>[2x]GPGGSPYLITGIPKDPKHPLPIRKDIDDWYLEQTSAGSNRIQLTLFVEALTVIQNRPLNDQLSYFRLAGIHGAPWTEWDGVPGGQKDSKGNPTGFAVHNNYTFPTWHRVYVTLYEQVIYEAMLDFIKQNVPQNGKADWENEAKQWRLPYWDFARFARHGHDNTQGDELRLPILVTMPMVKVLVPGQPGKQLSKPNPLYRFQMQTLMGTLERPYAITSQKTEEHGWSFDLPFDKCQSTTKYGLLENYNADVWADGGQNWLRANLALNEHPWYQNLDGWDSVPTLQDMTFRLLTTGGLNWGEFSSTRYDDKKEETQPKNNEQAPKNWMNLEAIHNNVHNWVGGFMFSRPGRHDLKLWGAGHMSSVPVAAYDPIFWLHHCNIDRLTAIWQTVNSGSWFNDDKSKVSKDDDLRPFHRFCEKTRKVVFFRSDDVKDWRSLNYDYAITKD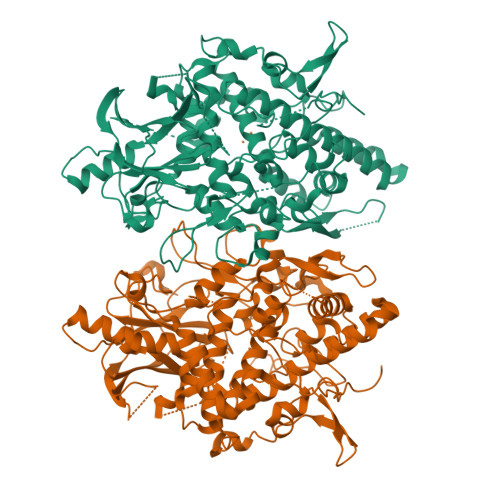ASRIRKEISDLYGQRTKEVYKDFGEEDYILSIRYSRYALGGKPFQINIFFGDVDGKDFYDARSQNFVGSVFNFSGSLEDSNCDKCAQQEQEGVLSVSQLPARLAVHYYKKQNKGEVPTPRYVVVNSQGKAEAEVKVEVALHKTEGTFYDAPARGGSDDYRRVADGKRAEVDDAYRA> MSREEVESLIQEVLEVYPEKARKDRNKHLAVNDPAVTQSKKCIISNKKSQPGLMTIRGCAYAGSKGVVWGPIKDMIHISHGPVGCGQYSRAGRRNYYIGTTGVNAFVTMNFTSDFQEKDIVFGGDKKLAKLIDEVETLFPLNKGISVQSECPIGLIGDDIESVSKVKGAELSKTIVPVRCEGFRGVSQSLGHHIANDAVRDWVLGKRDEDTT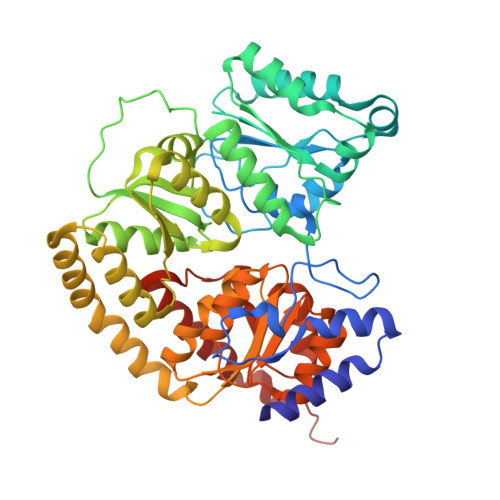FASTPYDVAIIGDYNIGGDAWSSRILLEEMGLRCVAQWSGDGSISEIELTPKVKLNLVHCYRSMNYISRHMEEKYGIPWMEYNFFGPTKTIESLRAIAAKFDESIQKKCEEVIAKYKPEWEAVVAKYRPRLEGKRVMLYIGGLRPRHVIGAYEDLGMEVVGTGYEFAHNDDYDRTMKEMGDSTLLYDDVTGYEFEEFVKRIKPDLIGSGIKEKFIFQKMGIPFREMHSWDYSGPYHGFDGFAIFARDMDMTLNNPCWKKLQAPWE> GPLGSMNDRADFVVPDITTRKNVGLSHDANDFTLPQPLDRYSAEDHATWATLYQRQCKLLPG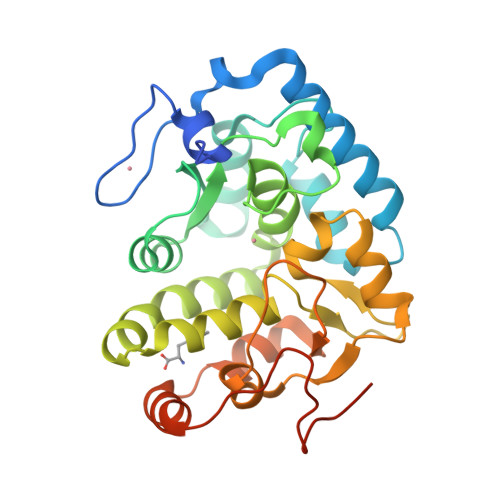RACDEFMEGLERLEVDADRVPDFNKLNQKLMAATGWKIVAVPGLIPDDVFFEHLANRRFPVTWWLREPHQLDYLQEPDVFHDLFGHVPLLINPVFADYLEAYGKGGVKAKALGALPMLARLYWYTVEFGLINTPAGMRIYGAGILSSKSESIYCLDSASPNRVGFDLMRIMNTRYRIDTFQKTYFVIDSFKQLFDATAPDFAPLYLQLADAQPWGAGDVAPDDLVLNAGDRQGWADTEDV>[3x]GAGTQTAQTQALDSDGIPTG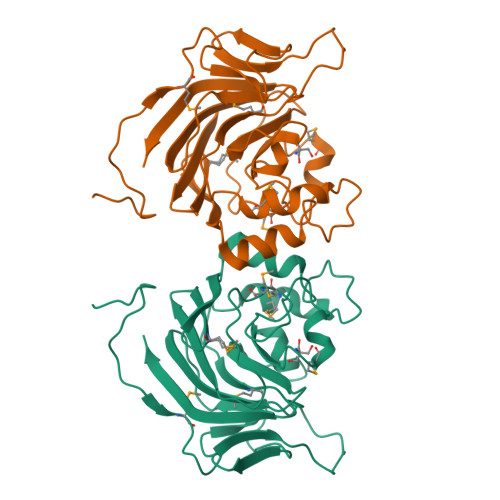GEWITMFDGKTLNGWRGYCRQDVPLGWVVEDGSITYKGSDNKADTGFGDLIYDKKFKNFVFEIEWKIDKAGNSGIFYTAQEIEGTPIYYSSPEYQLLDNENMPDAWEGCDGNRQAGAVYDMIMPDPQPVKPYGNWNKTRIVVYNQRVIHYMNDVKILEFQFGTPVWRALVDHSKFSKFSTSPEKCPEAYDLMLQCGKQPGYIGMQDHGYGVCFRNIRIKEL> MQRLFLLVAVMLLSGCLTAPPKEAARPTLMPRAQSYKDLTHLPAPTGKIFVSVYNIQDETGQFKPYPASNFSTAVPQSATAMLVTALKDSRWFIPLERQGLQ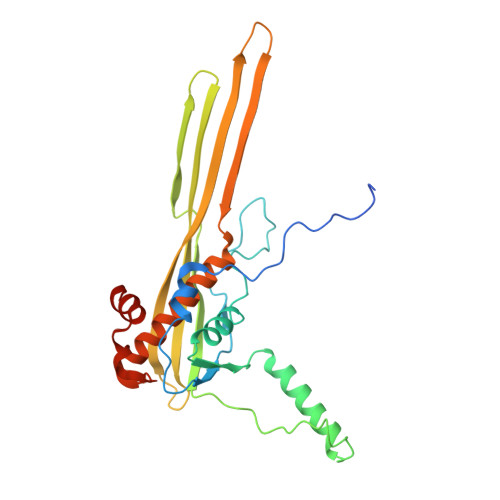NLLNERKIIRAAQENGTVAINNRIPLQSLTAANIMVEGSIIGYESNVKSGGVGARYFGIGADTQYQLDQIAVNLRVVNVSTGEILSSVNTSKTILSYEVQAGVFRFIDYQRLLEGEVGYTSNEPVMLCLMSAIETGVIFLINDGIDRGLWDLQNKAERQNDILVKYRHMSVPPES> SNAIMAKTAKVAVSQIVEHPALDATRQGLLDGLKAKGYEEGKNLEFDYKTAQGNPAIAVQIARQFVGENPDVLVGIATPTAQALVSATKTIPIVFTAVTDPVGAKLVKQLEQPGKNVTGLSDLSPVEQHVELIKEILPNVKSIGVVYNPGEANAVSLMELLKLSAAKHGIKLVEATALKSADVQSATQAIAEKSDVIYALIDNTVASAIEGMIVAAN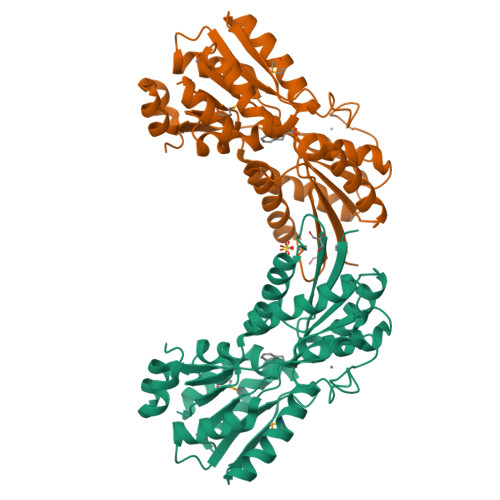QAKTPVFGAATSYVERGAIASLGFDYYQIGVQTADYVAAILEGKEPGSLDVQVAKGSDLVINKTAAEQLGITIPEAVLARATSTK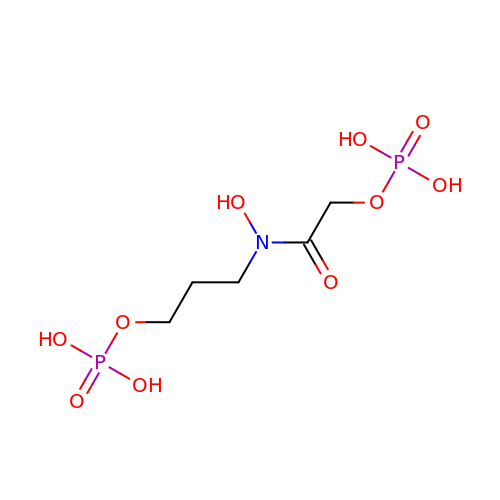3-{hydroxy[(phosphonooxy)acetyl]amino}propyl dihydrogen phosphate | C5 H13 N O10 P2 | IISKWLQYGVRJHI-UHFFFAOYSA-N>MPLLVEGRRVRLPQSAGDLVRAHPPLEERARLLRGQSVQQVGPQGLLYVQQRELAVTSPKDGSISILGSDDATTSHIVVLRHTGNGATCLTHCDGTDTKAEVPLIMNSIKSFSDHAQCGRLEVHLVGGFSDDRQLSQKLTHQLLSEFDRQEDDIHLVTLCVTELNDREENENHFPVIYGIAVNIKTAEIYRASFQDRGPEEQLRAARTLAGGPMISIYDAETEQLRIGPYSWTPFPHVDFWLHQDDKQILENLSTSPLAEPPHFV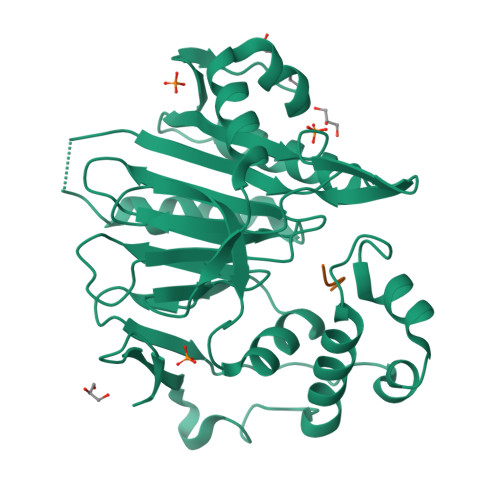EHIRSTLMFLKKHPSPAHTLFSGNKALLYKKNEDGLWEKISSPGSLEHHHHHH[2x];>NLAAR[2x]[(1R)-1-hydroxypropyl]phosphonic 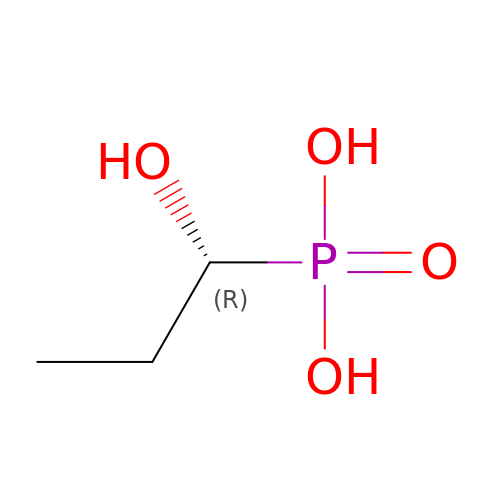acid | C3 H9 O4 P | MVIJUJBSAAUHEM-GSVOUGTGSA-N>MENKQKLKRPIQRIVRLSEEENNLIKRKIEESFFPNFQNFALHLLIQGEIRHVDYSELNRLTTEIHKIGININQMARLANQFHEISSEDIKDLTDKVQSLNALVQSELNKLIKRKDQS[4x]

The tetracycline-resistance plasmid pCF10 from E. faecalis is a member of the highly transmissible pheromone-responsive family of mobile genetic elements (MGEs) found in enterococci. PcfF binds to double stranded DNA (dsDNA) and is specific for inverted repeat sequences located within pCF10’s origin of transfer (oriT) sequence. PcfF-oriT complexes, however, recruit PcfG to form the relaxosome, as evidenced by supershifting of PcfF-oriT complexes in the presence of PcfG to higher molecular mass complexes in electrophoretic mobility shift assay (EMSA) experiments. Here, we have solved the structure of the accessory factor PcfF, which binds the pCF10 oriT sequence and recruits the PcfG relaxase for relaxosome assembly.

Crystals belonged to space group P21 and contained 4 molecules in the asymmetric unit. The structure was refined at a resolution of 1.9 Å. PcfF crystallized as a tetramer (dimer of dimers in a head to toe organization). However, the tetrameric interface is weak and deemed unstable by PISA calculations. The biologically relevant oligomer was suggested to be dimeric, in agreement with results from the SEC and GEMMA experiments. PcfF contains a RHH domain at the N terminus and a 2-helix bundle, here termed the stalk domain, at the C terminus. These two domains are connected by a hinge region. In the dimer, the RHH and stalk domains are built up by secondary structure elements from both monomers in the dimer. In agreement with findings from other RHH accessory factors, we determined that PcfF binds pCF10’s oriT sequence via its RHH-domain, and that mutation of the surface-exposed charged residues R13 and R16, as well as I14, in the β-sheet strongly abrogate oriT binding in vitro. We gained evidence that this patch mediates binding of PcfF to PcfG by showing that a single point mutation (I70S) abolishes PcfF-PcfG binding.> MEYFRYRGIIEGFYGKPWEHQERLDMFEFMQANNLNAYIYAPKQDLYHRELWREPYKEEQLQLFKELIEKAGSCGINFTFAISPGLSLVYSSEEELETLIRKITPFLEMGVHSIGIFFDNVPFDLIHEEDRNSYSNLAEAQADFLTRVLQRLESTISTPQIIMCPTFYCNDPNLEYLRILGQRLPKNIDVFWTGPNVCSHEITTSHMQEVQKSLQRPATLWDNYPVNDGGMMPELHIGPYDHRDPELHTHVVGIYANPMALPEASKLPLYTFAQYLNSPSQYNPQDSWRQAVSTLLGEDNLSAMEKFYQSNTISCLEPEEPAYLTNLFKKVQEDFASFRFEQGLRTLREEIISMQTTYSRLSTQDSKFFWEIRPWLEEYKLWTDYLDQAMITFSNLFTGFFTADEEQARESLQKALQGRTYLREVLKDAVDFRTRVCGDVVRNFLQQVLRSTVSIELQAEGKEWTALPPG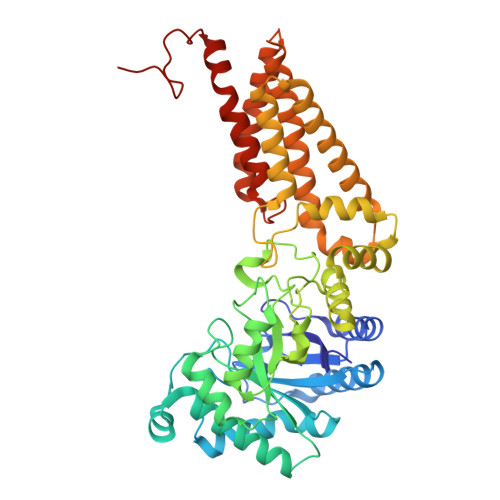IVRD>MSLSKKRKLESGDSGGAGAGGEGAEEENGGEQEAAPPRPRRTKSERDQLYYECYSDVSVHEEMIADQVRTEAYRLGILKNWAALRGKTVLDVGAGTGILSIFCAQAGARRVYAVEASAIWQQAREVVRLNGLEDRVHVLPGPVETVELPERVDAIVSEWMGYGLLHESMLSSVLHARTKWLKEGGLLLPASAELFVAPISDQMLEWRLGFWSQVKQHYGVDMSCMESFATRCLMGHSEIVVQDLSGEDVLARPQRFAQLELARAGLEQELEAGVGGRFRCSCYGSAPLHGFAVWFQVTFPGGDSEKPLVLSTSPLHPATHWKQALLYLNEPVPVEQDTDISGEITLLPSPDNPRRLRILLRYKVGDHEEKTKDFAMEDGSENLYFQG[2x]

Protein arginine methyltransferases (PRMTs) are important therapeutic targets, playing a crucial role in the regulation of many cellular processes and being linked to many diseases. Then, another series of compounds (12a–12h) were designed and synthesized, introducing also an adenosine moiety and exploring the distance between the three groups. We also report crystal structures with various PRMTs supporting the observed specificity and selectivity. On the contrary, we were able to cocrystallize the compounds in the complex with both PRMT4 and PRMT6.

Structure determinations and refinements revealed that only compounds 12a, 12c, and 12f are visible in the active site of each monomer of the PRMT6 dimer. In all the structures of the complexes with PRMT6, the electron density for the compound is always better in one monomer. Compound 12a is the only one for which a complete electron density is visible in one monomer of the PRMT6 structure, whereas for 12c and 12f the electron density becomes fragmented after the guanidine group and the density for the methyl-4-hydroxy-2-naphthoate moiety is weak. The crystal structure revealed an unusual distorted U-shaped conformation adopted by compound 12a (and probably also 12c and 12f) in the binding to PRMT6, with a folding at the level of the guanidine group. Whereas the adenosine moiety lies into its canonic binding pocket, the guanidine group of the compounds is unable to reach the PRMT6 double-E loop clamp because the linker with the sugar is too short, even for the longer compound 12f. Instead of binding in the arginine substrate pocket as observed with PRMT4, the methyl-4 hydroxy-2-naphthoate moiety is sandwiched between the adenosine and the side chains of Y50 and Y51 residues of the α helix motif I. Hence, the binding of compounds 12a, 12c, and 12f affects the proper folding of the PRMT6 alpha-X helix containing the motif I (Y50-Y51-X-X-Y54).> MAHHHHHHMLPIQKKVGYLIKDDSEKQATITNTKYSTLANPYISVANIMLQNYVKQREKYNYDTLKEQFTFIKNASTSIVYMQFANFMNIDNSLSPVIR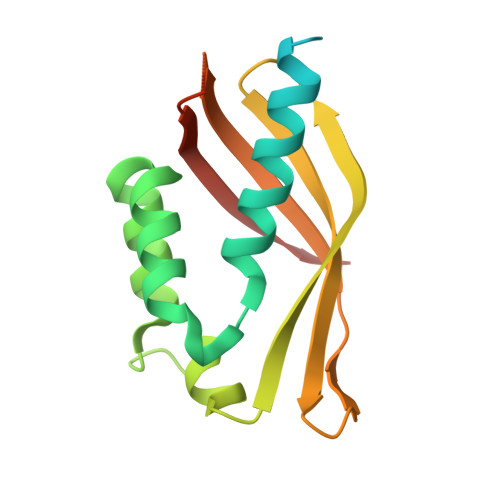YQKLYRRSINIISINNINNNEATVTFESLAQNNTGEILENMLWEAKIGFIMDSISTSTLHNMPFHFIVTSYKLKLLRNKNQQ> GPYTFVQQHLMIGTDPRTILKDLLPETIPPPELDDMTLWQIVINILSEPPKRKKRKDINTIEDAVKLLQECKKIIVLTGAGVSVSCGIPDFRSRDGIYARLAVDFPDLPDPQAMFDIEYFRKDPRPFFKFAKEIYPGQFQPSLCHKFIALSDKEGKLLRNYTQNIDTLEQVAGIQRIIQCHGSFATASCLICKYKVDCEAVRGDIFNQVVPRCPRCPADEPLAIM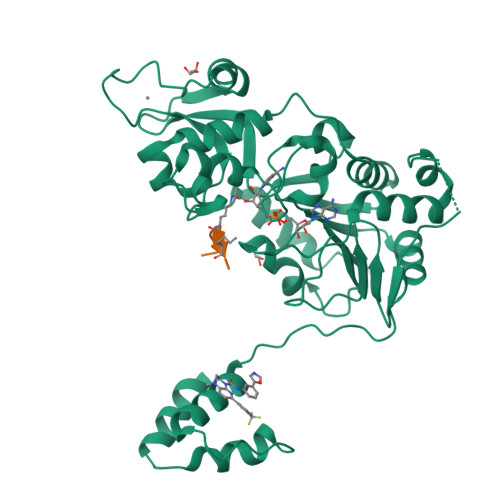KPEIVFFGENLPEQFHRAMKYDKDEVDLLIVIGSSLKVRPVALIPSSIPHEVPQILINREPLPHLHFDVELLGDCDVIINELCHRLGGEYAKLCCNPVGGGSGGGSQYLFLPPNRYIFHGAEVYSDSEDDV;> RHKKLLF The very first step of this initiation process is accomplished by DNA association with the Origin Recognition Complex (ORC), a six-subunit protein that forms a partial ring around origin DNA. The complex consists of six subunits (ORC1-6), with subunits ORC1-5 forming a partial ring capable of encircling DNA. All five subunits contain a winged-helix domain (WHD) and a AAA+ domain which consists of the RecA-fold and lid domains, although the ORC2 and ORC3 RecA-folds have diverged slightly and do not contain a lid domain. Adjacent ORC subunits associate in a double-layer arrangement through interfaces between the WHDs in one layer and the AAA+ domains in another with ATP-binding sites sandwiched between the ORC1·4, ORC4·5, and ORC5·3 AAA+ interfaces (Tocilj et al., 2017).

The first of these, ORCO2WH, consists of a dynamic ORC1 AAA+ domain that is unresolved in the refined map. Interestingly, in this structure, the ORC2 WHD was stably bound inside the ring-shaped core of ORC in a conformation that is similar to the auto-inhibited state observed in the DmORC structure (Bleichert et al., 2015). Only in the ORCO2WH structure was an ATP absent at the ORC1·4 site due to the displacement of the ORC1 AAA+-domain and consequential disruption of the ATP binding site. In contrast, in the ORCO2WH structure, the ORC1 AAA+ rotates ~90° from a position proximal to the ORC4 AAA+ domain where it completes the major ATP binding site in the ORCO1AAA structure, to a position proximal to the ORC1 and ORC5 WHDs, disrupting the ORC1·4 ATP binding site. The latter position resembles the auto-inhibited state observed in the DmORC structure. A minor ORC2 WHD conformation was observed in further 3D classifications of the ORCO2WH particles. In fact, this conformation resembles the completely collapsed ORC2 WHD conformations in the ORCO2-5 structure where the domain is further tucked into the core of the complex compared to the auto-inhibited state. Notably, this alternative conformation does not resemble any of the conformations of ORC2 WHD in any previously reported structures of the various ORCs. Overall, the ORCO1AAA and ORCO2WH populations reveal a dynamic switch between the ORC1 AAA+ and ORC2 WHD where the locking into position of one domain within the ORC ring-shaped core kicks the other domain into a dynamic state.

> MAPQIRSRSLAAQEPASVLEEARLRLHVSAVPESLPCREQEFQDIYNFVESKLLDHTGGCMYISGVPGTGKTATVHEVIRCLQQAAQANDVPPFQYIEVNGMKLTEPHQVYVQILQKLTGQKATANHAAELLAKQFCTRGSPQETTVLLVDELDLLWTHKQDIMYNLFDWPTHKEARLVVLAIANTMDLPERIMMNRVSSRLGLTRMCFQPYTYSQLQQILRSRLKHLKAFEDDAIQLVARKVAALSGDARRCLDICRRATEICEFSQQKPDSPGLVTIAHSMEAVDEMFSSSYITAIKNSSVLEQSFLRAILAEFRRSGLEEATFQQIYSQHVALCRMEGLPYPTMSETMAVCSHLGSCRLLLVEPSRNDLLLRVRLNVSQDDVLYALKDE;> MSKPELKEDKMLEVHFVGDDDVLNHILDREGGAKLKKERAQLLVNPKKIIKKPEYDLEEDDQEVLKDQNYVEIMGRDVQESLKNGSATGGGNKVYSFQNRKHSEKMAKLASELAKTPQKSVSFSLKNDPEITINVPQSSKGHSASDKVQPKNNDKSEFLSTAPRSLRKRLIVPRSHSDSESEYSASNSEDDEGVAQEHEEDTNAVIFSQKIQAQNRVVSAPVGKETPSKRMKRDKTSDLVEEYFEAHSSSKVLTSDRTLQKLKRAKLDQQTLRNLLSKVSPSFSAELKQLNQQYEKLFHKWMLQLHLGFNIVLYGLGSKRDLLERFRTTMLQDSIHVVINGFFPGISVKSVLNSITEEVLDHMGTFRSILDQLDWIVNKFKEDSSLELFLLIHNLDSQMLRGEKSQQIIGQLSSLHNIYLIASIDHLNAPLMWDHAKQSLFNWLWYETTTYSPYTEETSYENSLLVKQSGSLPLSSLTHVLRSLTPNARGIFRLLIKYQLDNQDNPSYIGLSFQDFYQQCREAFLVNSDLTLRAQLTEFRDHKLIRTKKGTDGVEYLLIPVDNGTLTDFLEKEEEEA;> MATSSMSKGCFVFKPNSKKRKISLPIEDYFNKGKNEPEDSKLRFETYQLIWQQMKSENERLQEELNKNLFDNLIEFLQKSHSGFQKNSRDLGGQIKLREIPTAALVLGVNVTDHDLTFGSLTEALQNNVTPYVVSLQAKDCPDMKHFLQKLISQLMDCCVDIKSKEEESVHVTQRKTHYSMDSLSSWYMTVTQKTDPKMLSKKRTTSSQWQSPPVVVILKDMESFATKVLQDFIIISSQHLHEFPLILIFGIATSPIIIHRLLPHAVSSLLCIELFQSLSCKEHLTTVLDKLLLTTQFPFKINEKVLQVLTNIFLYHDFSVQNFIKGLQLSLLEHFYSQPLSVLCCNLPEAKRRINFLSNNQCENIRRLPSFRRYVEKQASEKQVALLTNERYLKEETQLLLENLHVYHMNYFLVLRCLHKFTSSLPKYPLGRQIRELYCTCLEKNIWDSEEYASVLQLLRMLAKDELMTILEKCFKVFKSYCENHLGSTAKRIEEFLAQFQSLDAETKEEEDASGSQPKGLQKTDLYHLQKSLLEMKELRRSKKQTKFEVLRENVVNFIDCLVREYLLPPETQPLHEVVYFSAAHALREHLNAAPRIALHTALNNPYYYLKNEALKSEEGCIPNIAPDICIAYKLHLECSRLINLVDWSEAFATVVTAAEKMDANSATSEEMNEIIHARFIRAVSELELLGFIKPTKQKTDHVARLTWGGC;> MSSRKSKSNSLIHTECLSQVQRILRERFCRQSPHSNLFGVQVQYKHLSELLKRTALHGESNSVLIIGPRGSGKTMLINHALKELMEIEEVSENVLQVHLNGLLQINDKIALKEITRQLNLENVVGDKVFGSFAENLSFLLEALKKGDRTSSCPVIFILDEFDLFAHHKNQTLLYNLFDISQSAQTPIAVIGLTCRLDILELLEKRVKSRFSHRQIHLMNSFGFPQYVKIFKEQLSLPAEFPDKVFAEKWNENVQYLSEDRSVQEVLQKHFNISKNLRSLHMLLMLALNRVTASHPFMTAVDLMEASQLCSMDSKANIVHGLSVLEICLIIAMKHLNDIYEEEPFNFQMVYNEFQKFVQRKAHSVYNFEKPVVMKAFEHLQQLELIKPMERTSGNSQREYQLMKLLLDNTQIMNALQKYPNCPTDVRQWATSSLSWL;> MPHLENVVLCRESQVSILQSLFGERHHFSFPSIFIYGHTASGKTYVTQTLLKTLELPHVFVNCVECFTLRLLLEQILNKLNHLSSSEDGCSTEITCETFNDFVRLFKQVTTAENLKDQTVYIVLDKAEYLRDMEANLLPGFLRLQELADRNVTVLFLSEIVWEKFRPNTGCFEPFVLYFPDYSIGNLQKILSHDHPPEYSADFYAAYINILLGVFYTVCRDLKELRHLAVLNFPKYCEPVVKGEASERDTRKLWRNIEPHLKKAMQTVYLREISSSQWEKLQKDDTDPGQLKGLSAHTHVELPYYSKFILIAAYLASYNPARTDKRFFLKHHGKIKKTNFLKKHEKTSNHLLGPKPFPLDRLLAILYSIVDSRVAPTANIFSQITSLVTLQLLTLVGHDDQLDGPKYKCTVSLDFIRAIARTVNFDIIKYLYDFL> MAQILPIRFQEHLQLQNLGINPANIGFSTLTMESDKFICIREKVGEQAQVVIIDMNDPSNPIRRPISADSAIMNPASKVIALKAGKTLQIFNIEMKSKMKAHTMTDDVTFWKWISLNTVALVTDNAVYHWSMEGESQPVKMFDRHSSLAGCQIINYRTDAKQKWLLLTGISAQQNRVVGAMQLYSVDRKVSQPIEGHAASFAQFKMEGNAEESTLFCFAVRGQAGGKLHIIEVGTPPTGNQPFPKKAVDVFFPPEAQNDFPVAMQISEKHDVVFLITKYGYIHLYDLETGTCIYMNRISGETIFVTAPHEATAGIIGVNRKGQVLSVCVEEENIIPYITNVLQNPDLALRMAVRNNLAGAEELF;> SQPLI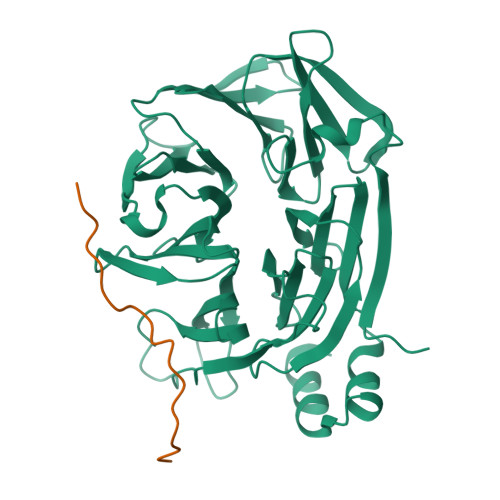DLPLIDFCDTPEAHVAVGSESRPLIDLMTNTPDMNKNVAKPSPVVGQLIDLSSPLIQLSPE> MRVWVGIDDTDSSRGMCTTYLAVLAMERVERELGKVIGFPRLIRLNPTIPYKTRGNGAVSFLVEVDDVGELVDVVNEVIIEHAMLDDEKTNPGAVFVDEELAVKLKPFADKAIKDVLQIDEALFVIGKYFIPHLRHKKGRGLIGALAAVGAELEDFTLELIAYRYPERFGTEREYDEESFFDMDYELYPQTFDNVDWCNDVVVCIPNTPCPVLYGIRGESVEALYKAMESVKTEPVDRRMIFVTNHATDMHLIGEEEVHRLENYRSYRLRGRVTLEPYDIEGGHVFFEIDTKFGSVKCAAFEPTKQFRNVIRLLRKGDVVEVYGSMKKDTINLEKIQI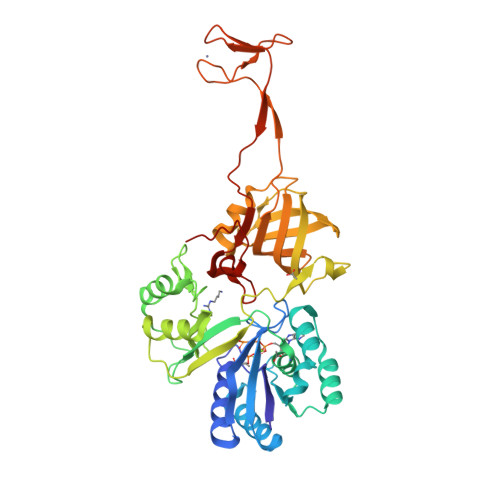VELAEIWVEKNPICPSCGRRMESAGRGQGFRCKKCRTKADEKLREKVERELQPGFYEVPPSARRHLSKPLIRMNVEGRHIFR>PY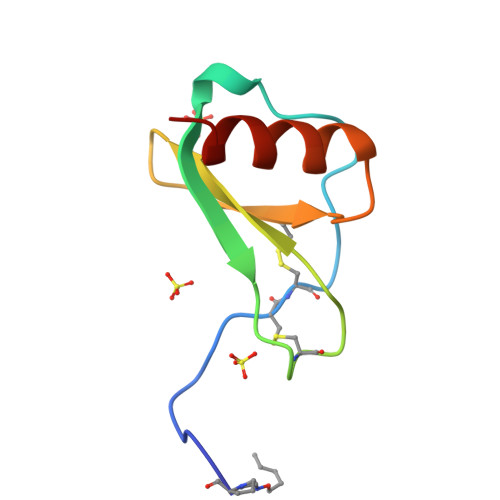SSDTTPCCFAYIARPLPRAHIKEYFYTSGKCSNPAVVFVTRKNRQVCANPEKKWVREYINSLEMS[2x]> GIDPFTMADDLPPAPVITAQASVPLTSESFVAAAVSRSGPAVVRIDTETVVTRRTDPILDDPFFQEFFGRSFPVPPRERRIAGQGSGFIIDNSGIILTNAHVVDGASKVVVTLRDGRTFDGQVRGTDEVTDLAVVKIEPQGSALPVAPLGTSSNLQVGDWAIAVGNPVGLDNTVTLGIISTLGRSAAQAGIPDKRVEFIQTDAAINPGNAGGPLLNARGEVIGINTAIRADATGIGFAIPIDQAKAIQNTLAAGGTVPHPYIGVQMMNITVDQAQQNNRNPNSPFIIPEVDGILVMRVLPGT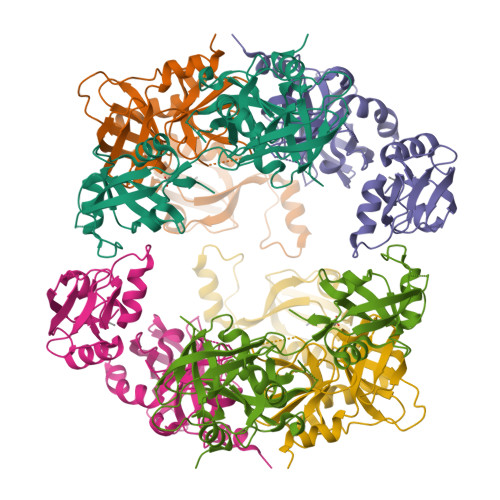PAERAGIRRGDVIVAVDGTPISDGARLQRIVEQAGLNKALKLDLLRGDRRLSLTVQTAQLRNPTS> MHHHHHHMLPRDCQELFQVGERQSGLFEIQPQGSPPFLVNCKMTSDGGWTVIQRRHDGSVDFNRPWEAYKAGFGDPHGEFWLGLEKVHSITGDRNSRLAVQLRDWDGNAELLQFSVHLGGEDTAYSLQLTAPVAGQLGATTVPPSGLSVPFSTWDQDHDLRRDKNCAKSLSGGWWFGTCSHSNLNGQYF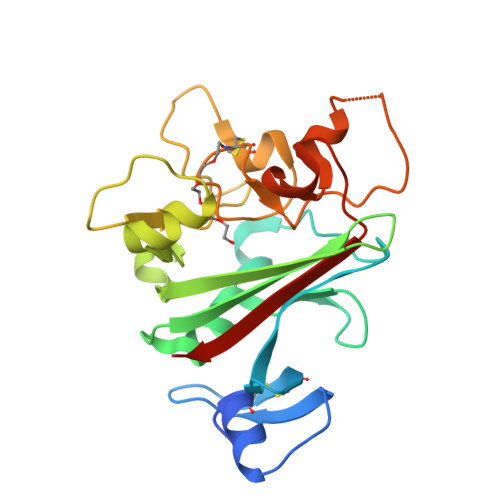RSIPQQRQKLKKGIFWKTWRGRYYPLQATTMLIQPMAAEAAS>[8x]MVSKGEEDNMASLPATHELHIFGSINGVDFDMVGQGTGNPNEGYEELNLKSTKGDLQF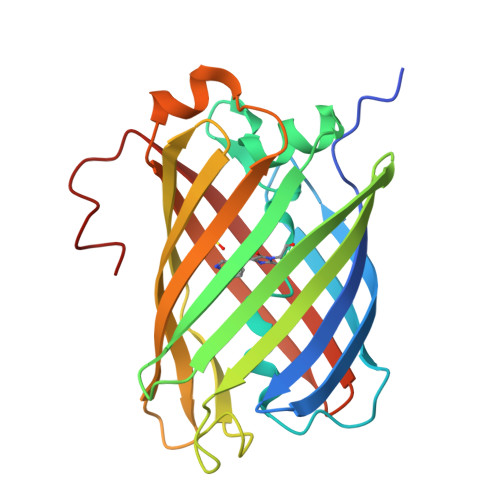SPWILVPHVGWGFHQYLPYPDGMSPFQAAMVDGSGYQVHRTMQFEDGASLTVNYRYTYEGSHIKGEAQVKGTGFPADGPVMTNSLTAVDSCWSKKTYPNDKTIISTFKWSYTTGNGERYRSTARTTYTFAKPMAANYLKNQPVYVFRKTELKHSETELNFKEWQKAFTDVMGMDELYK> NGFPWVIVVGPI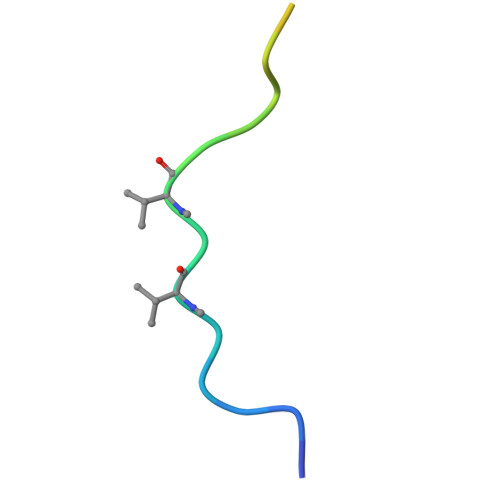GVIGSVMSTE>[2x]PQDVDFHIPLPGRQSPDHARAEAEQLAWPRSLGLIRSDAAAERHLRGGYADLASRFYP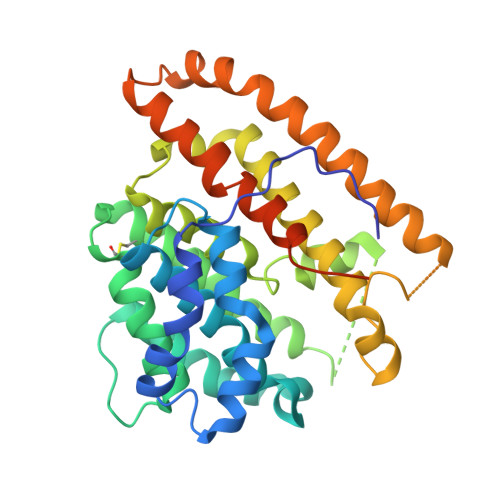HATGADLDLGVDLMSWFFLFDDLFDGPRGENPEDTKQLTDQVAAALDGPLPDTAPPIAHGFADIWRRTCEGMTPAWCARSARHWRNYFDGYVDEAESRFWNAPCDSAAQYLAMRRHTIGVQPTVDLAERAGRFEVPHRVFDSAVMSAMLQIAVDVNLLLLDIASLEKEEARGEQNNMVMILRREHGWSKSRSVSHMQNEVRARLEQYLLLESCLPKVGEIYQLDTAEREALERYRTDAVRTVIRGSYDWHRSSGRYDAEFALAAGAQGYLEELGSSAH> ETGVALEQRPISITRNAKQSASLNCKILNPVSDYVHWYRSQEGRAPERLLVYSRSKSESVPDPGFSADKVRAYKGKDDTCRLIVSDLQVSDSGVYHCASWDGRVKVFGEGTRLIVTESAFKKKPPKPIFFLPTSEEIKQKQSGTYICLLEDFFPNVVKTYWKEDGNSQPLDAQFGPITGGGNSYS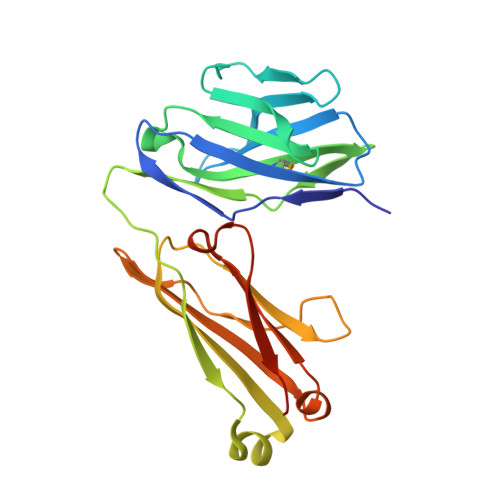QVSWLTVKEDVLRKNLTYFYQHEDLGMEPKAFSISSVREKGSLVPR> PGPPGIVIVEEITESTATLSWSPAADNHSPISSYNLQARSPFSLGWQTVKTVPEIITGDMESAMAVDLNPWVEYEFRVVATNPIGTGDPSTPSRMIRTNEAVPKTAPTNVSGRSGRRHELVIAWEPVSEEFQNGEGFGYIVAFRPNGTRGWKEKMVTSSEASKFIYRDESVPPLTP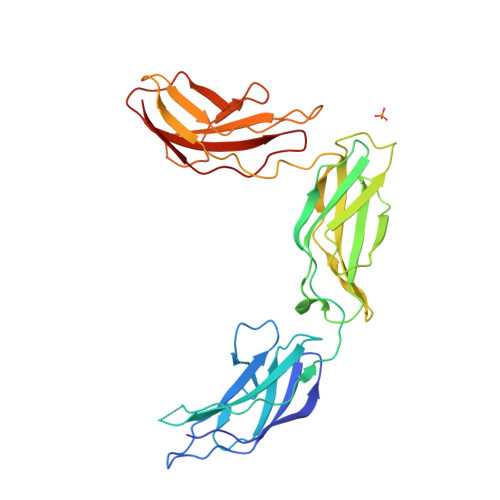FEVKVGVYNNKGDGPFSQIVVICSAEGEPSAAPTDVKATSVSVSEILVAWKHIKESLGRPQGFEVGYWKDMEQEDTAETVKTRGNESFVILTGLEGNTLYHFTVRAYNGAGYGPPSSEVSATT>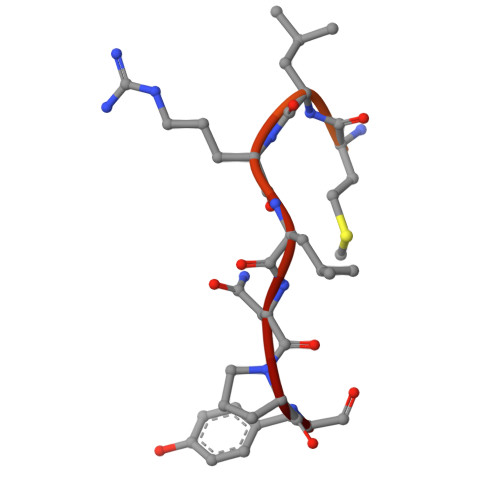 SRTKRACVQKKNPLRNKQIMLRLNPY> MSLIYTITLNPAIDRL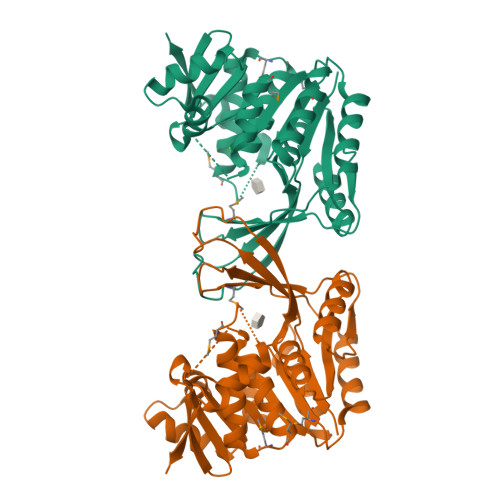LFIRGELEKRKTNRVIKTEFDCGGKGLHVSGVLSKFGIKNEALGIAGSDNLDKLYAILKEKHINHDFLVEAGTSTRECFVVLSDDTNGSTMIPEAGFTVSQTNKDNLLKQIAKKVKKEDMVVIAGSPPPHYTLSDFKELLRTVKATGAFLGCDNSGEYLNLAVEMGVDFIKPNEDEVIAILDEKTNSLEENIRTLAEKIPYLVVSLGAKGSICAHNGKLYQVIPPKVQERNDTGAGDVFVGAFIAGLAMNMPITETLKVATGCSASKVMQQDSSSFDLEAAGKLKNQVSIIQLEEREGHHHHHH> GPLGSNPASLYRIDLFITFTDELITFDYKVHGRPVLTFRIPGFGLTPAGRMLVCMGEKPAHSPFTSSKSLYHVIFTSTCNSFSFTIYKGRYRSWKKPIHDELVDRGYTTFREFFKAVRGYHADYYKQRLIHDVEMNPG

The 2A protein of Theiler's murine encephalomyelitis virus (TMEV) acts as a switch to stimulate programmed –1 ribosomal frameshifting (PRF) during infection. Secondly, the viral 2A protein is required as a trans-activator of frameshifting in cells and in vitro which permits temporally controlled, variable-efficiency frameshifting related to the amount of 2A protein in the cell during infection. Our previous investigations of protein-stimulated frameshifting in EMCV and TMEV have revealed that the viral 2A protein acts in complex with a stem-loop downstream of the slippery sequence, and that this interaction can be disabled by mutating either a conserved cytosine triplet in the loop or a pair of conserved arginine residues in the protein. Despite highly divergent sequences within cardioviruses, the TMEV 2A protein adopts the second known occurrence of the beta-shell fold.

We crystallised the protein but were unable to solve the structure by molecular replacement using the crystal structure of the closest homologue, EMCV 2A, as a search model. Instead, we obtained experimental phases via bromine derivatisation and determined the structure by single-wavelength anomalous dispersion analysis. The asymmetric unit of the cubic cell contained a single copy of 2A, which was refined to 1.9 Å resolution. Interpretable electron density was visible for 2A residues 1–126, with a short G-4P-3L-2G-1S0 N-terminal extension that resulted from 3C protease cleavage of the GST tag. In the crystalline lattice these residues mediate contacts between symmetry-related molecules, consistent with recombinant 2A forming trimers at high concentrations. Since tag-derived residues mediate the inter-subunit contacts, the 2A trimerisation interface that we observe in crystallo is unlikely to be physiologically relevant. The structure of TMEV 2A reveals a globular β3αβ3α fold, with a similar ‘beta-shell’ architecture to EMCV 2A (Cα backbone RMSD of 2.65 Å over 130 residues). An extensive curved antiparallel six-stranded beta sheet packs against two alpha helices on the concave surface of the sheet, whilst the loops between adjacent beta strands project from the opposite convex face. At physiological pH the protein will thus have a positive electrostatic surface potential across the convex face of the beta sheet, surrounding loops and the N-terminal end of helix α1, suggesting a putative RNA-binding surface. Conversely, in TMEV 2A, the α2 helix continues with a pronounced 90° kink until the end of the protein.> MRGSHH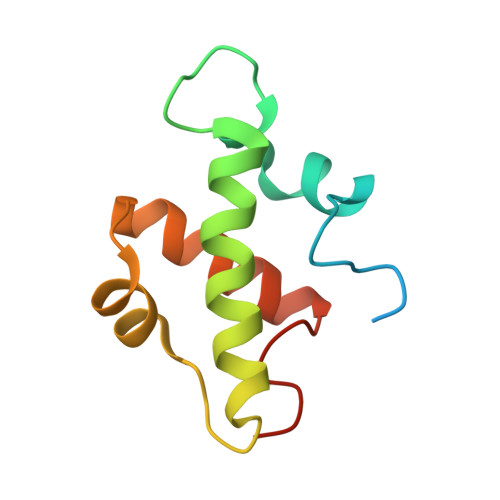HHHHGMASSYSKWFNLEKIHSIEVQSLPEFFTNRIPSKTPEVYMRYRNFMVNSYRLNPNEYFSVTTARRNVSGDAAALFRLHKFLTKWGLINYQVDSK>[2x]MPGLFLTLEGLDGSGKTTQARRLAAFLEAQGRPVLLTREPGGGLPEVRSLLLTQELSPEAEYLLFSADRAEHVRKVILPGLAAGKVVISDRYLDSSLAYQGYGRGLPLPW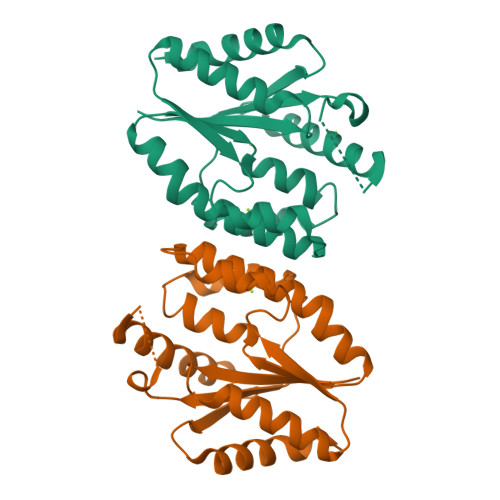LREVAREATRGLKPRLTFLLDLPPEAALRRVRRPDRLEGLGLEFFRRVREGFLALARAEPGRFVVLDATLPEEEIARAIQAHLRPLLP>[3x]AEPFAKLEQDFGGSIGVYAMDTGSGAT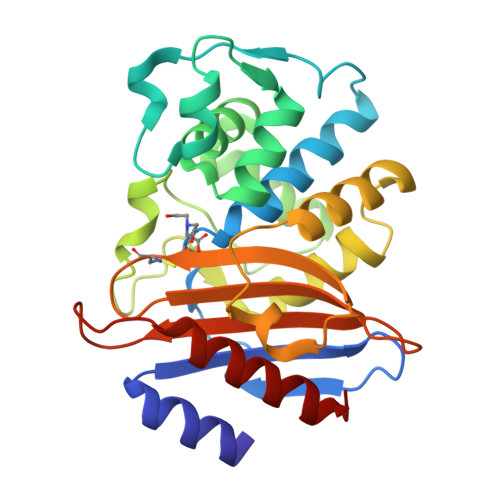VSYRAEERFPLCSSFKGFLAAAVLARSQQQAGLLDTPIRYGKNALVPWSPISEKYLTTGMTVAELSAAAVQYSDNAAANLLLKELGGPAGLTAFMRSIGDTTFRLDRWELELNSAIPGDARDTSSPRAVTESLQKLTLGSALAAPQRQQFVDWLKGNTTGNHRIRAAVPADWAVGDKTGTCGVYGTANDYAVVWPTGRAPIVLAVYTRAPNKDDKHSEAVIAAAARLALEGLGV>MFERFTDRARRVVVLAQEEARMLNHNYIGTEHILLGLIHEGEGVAAKSLESLGISLEGVRSQVEEIIGQGQQAPSGHIPFTPRAKKVLELSLREALQLGHNYIGTEHILLGLIREGEGVAAQVLVKLGAELTRVRQQVIQLLSGYQGKEAAEAGTGGRGGESGSPSTSLVLDQFGRNLTAAAMEGKLDPVIGREKEIERVMQVLSRRTKNNPVLIGEPGVGKTAVVEGLAQAIVHGEVPETLKDKQLYTLDLGSLVAGSRYRGDFEERLKKVLKEINTRGDIILFIDELHTLVGAG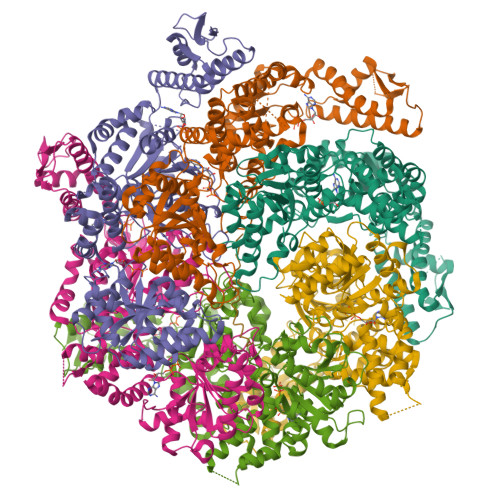AAEGAIDAASILKPKLARGELQTIGATTLDEYRKYIEKDAALERRFQPVQVGEPTVEHTIEILKGLRDRYEAHHRVSITDAAMVAAATLADRYINDRFLPDKAIDLIDEAGARMRIRRMTAPPDLREFDEKIAEARREKESAIDAQDFEKAASLRDREKTLVAQRAEREKQWRSGDLDVVAEVDDEQIAEVLGNWTGIPVFKLTEAETTRLLRMEEELHKRIIGQEDAVKAVSKAIRRTRAGLKDPKRPSGSFIFAGPSGVGKTELSKALANFLFGDDDALIQIDMGEFHDRFTASRLFGAPPGYVGYEEGGQLTEKVRRKPFSVVLFDEIEKAHQEIYNSLLQVLEDGRLTDGQGRTVDFKNTVLIFTSNLGTSDISKPVGLGFSKGGGENDYERMKQKVNDELKKHFRPEFLNRIDDIIVFHQLTREEIIRMVDLMISRVAGQLKSKDMALVLTDAAKALLAKRGFDPVLGARPLRRTIQREIEDQLSEKILFEEVGPGQVVTVDVDNWDGEGPGEDAVFTFTGTRKPPAEPDLAKAGAHSAGGPEPAARLEHHHHHH[6x]>[7x]MRLEDLQEELKKDVFIDSTKLQYEAANNVMLYSKWLNKHSSIKKEMLRIEAQKKVALKARLDYYSGRGDGDEFSMDRYEKSEMKTVLSADKDVLKVDTSLQYWGILLDFCSGAL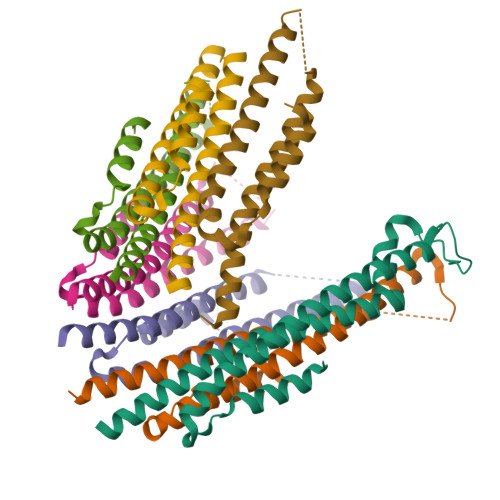DAIKSRGFAIKHIQDMRAFEAGK> MSYQSTIVPVELH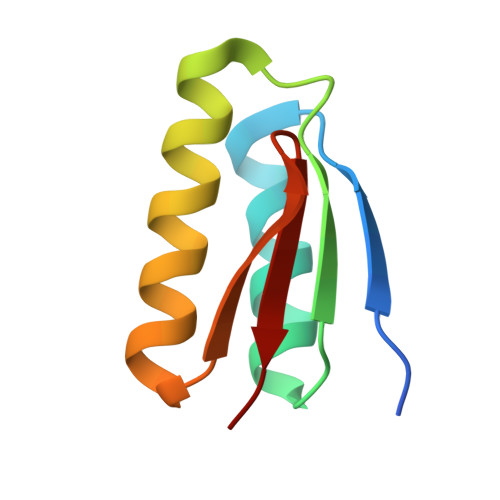SFEDAQVIGGAFRDGDAVVFDMSLLSREEARRIVDFAAGLCFALRGKMQKIDSVTFAVVPE>GSHMRNVAAEQQLRELESTFDGRLGFVALDTATGARIAHRADERFPFCSTFKTMLSAAVLARSAGDAALLQRRIPYAKRDLVRYSPITEKHVGAGMTVAELCAATLQYSDNTAADLLIALLGGPQAVTAYARSIGDATFRLDRRETELNTAIPGDERDTTTPAA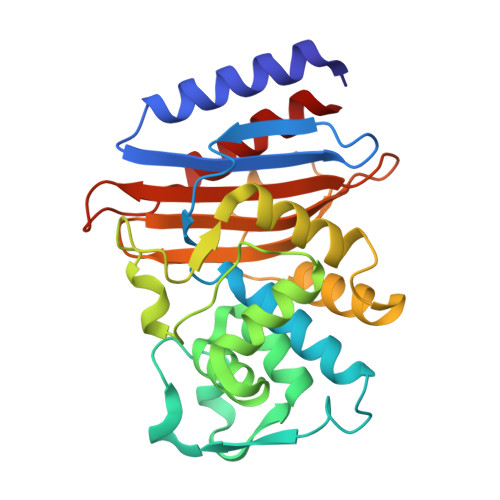MAASVRRLLVGDALGTAQRAQLNAWMLGNKTGDARIRAGVPAGWRVADKTGTGDYGTGNDIGVAYPPDRAPIVFVVYTTMRSRNAQARDDVIASAARIAARAFV[2x]>[4x]MNKDIASASNNNQNITNYSIEENIINLKYKIRKNAVKKINTEREIQQLSNNDP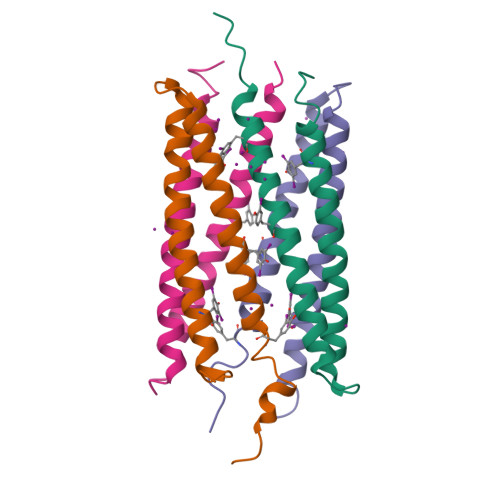NKNTLLALKQNLENLIHNQKEQLKTYQKLLKTLNDENN>ETGNYANGKNNVPRLKLSYKEMLESNNVITFNGLANSSSYHTFLLDEERSRLYVGAKDHIFSFNLVNIKDFQKIVWPVSYTRRDECKWAGKDILKECANFIKVLEAYNQTHLYACGTGAFHPICTYIEVGHHPEDNIFKLQDSHFENGRGKSPYDPKLLTASLLIDGELYSGTAADFMGRDFAIFRTLGHH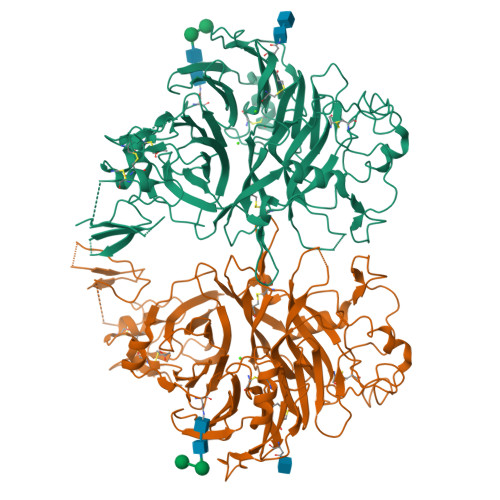HPIRTEQHDSRWLNDPRFISAHLIPESDNPEDDKVYFFFRENAIDGEHSGKATHARIGQICKNDFGGHRSLVNKWTTFLKARLICSVPGPNGIDTHFDELQDVFLMNSKDPKNPIVYGVFTTSSNIFKGSAVCMYSMSDVRRVFLGPYAHRDGPNYQWVPYQGRVPYPRPGTCPSKTFGGFDSTKDLPDDVITFARSHPAMYNPVFPINNRPIMIKTDVNYQFTQIVVDRVDAEDGQYDVMFIGTDVGTVLKVVSVPKETWHDLEEVLLEEMTVFREPTTISAMELSTKQQQLYIGSTAGVAQLPLHRCDIYGKACAECCLARDPYCAWDGSSCSRYFPTAKARTRAQDIRNGDPLTHCSDXXXXXXXXXXXXXXXXXXXXXXXXXXXXXXXXXXXXXXXXXXXXXXXXXXXXXXXXXXXXXXXXXXXXXXXXXXXXXXXXXXXXXXXXXXXXXXXXXXXXXXXXXXXXXXXXXXX[2x]> MENKTPIFFSLSIFLSLLNCAEAGNDLLSCLTFNGVRNHTVFSADSDSDFNRFLHLSIQNPLFQNSLISKPSAIILPGSKEELSNTIRCIRKGSWTIRLRSGGHSYEGLSYTSDTPFILIDLMNLNRVSIDLESETAWVESGSTLGELYYAITESSSKLGFTAGWCPTVGTGGHISGGGFGMMSRKYGLAADNVVDAILIDANGAILDRQAMGEDVFWAIRGGGGGVWGAIYAWKIKLLPVPEKVTVFRVTKNVAIDEATSLLHKWQFVAEELEEDFTLSVLGGADEKQVWLTMLGFHFGLKTVAKSTFDLLFPELGLVEEDYLEMSWGESFAYLAGLETVSQLNNRFLKFDERAFKTKVDLTKEPLPSKAFYGLLERLSKEPNGFIALNGFGGQMSKISSDFTPFPHRSGTRLMVEYIVAWNQ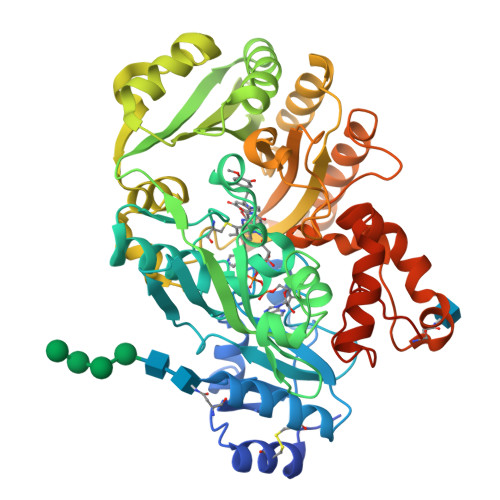SEQKKKTEFLDWLEKVYEFMKPFVSKNPRLGYVNHIDLDLGGIDWGNKTVVNNAIEISRSWGESYFLSNYERLIRAKTLIDPNNVFNHPQSIPPMANFDYLEKTLGSDGGEVVI(2~{S})-2-acetamido-~{N}-(3-bromanylprop-2-ynyl)propanamide | C8 H11 Br N2 O2 | 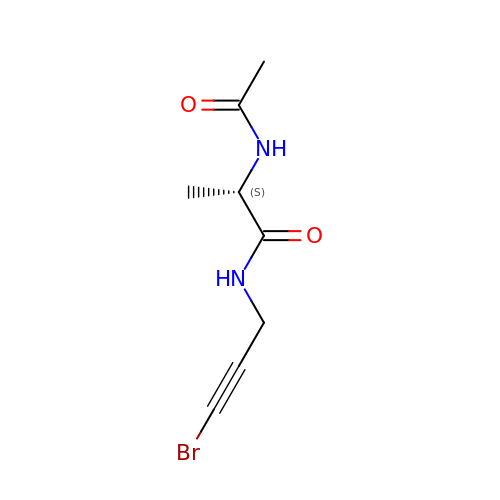LBAQBIGJPXWVEB-LURJTMIESA-N> NVDEFLFISNNFKQYKEFIDMD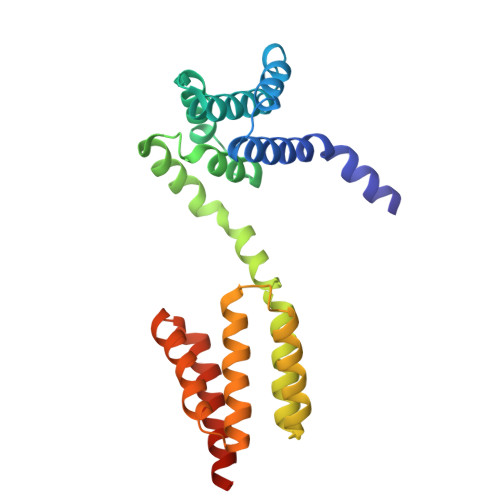TAKHYFECRNIEGLNHILDSYKDSKSTKEKNLFALVKVLLATLTEEDCLTERTYLSNYLINIETWSHYETVLFNNCMFIFESCFIEMVFSKVILNLDKYNTLRYYGNESIRMFVNMLILFIQRQEYDKASEILAKIEDYQLNDDCLYERCCVSFFDGIIGLINGKEGAEQKCVQILEIFQLLNCKTIHHMFQTYLEAIKHKLSLEHHHHHH The soluble glucose dehydrogenase (sGDH) from Acinetobacter calcoaceticus has been widely studied and is used, in biosensors, to detect the presence of glucose, taking advantage of its high turnover and insensitivity to molecular oxygen. However, this dimeric enzyme, composed of two identical 453 amino acid monomers (pI = 8.75), also presents drawbacks in terms of broad substrate specificity and loss of activity over time. Briefly, all crystal structures contained a tight dimer of sGDH in the asymmetric unit, the dimeric interface extending over 1110 Å2 being maintained by the presence of two calcium ions as described in Oubrie et al. interacting with the N262-D273 loop, referred to as the 4CD loop in the nomenclature of Oubrie et al.. 2Fobs-Fcalc electron density maps from the wild-type and both mutant structures all showed a different molecule instead of the PQQ-cofactor, corresponding to a PQQ modified cofactor, with the bond between C4 and C5 missing.

The active site of PQQ from the wild-type enzyme at pH 8. The density at 5 σ from a Polder Omit Map (PHENIX) is superimposed onto a model of cleaved PQQ. Residues close to the cofactor are labeled, and show little reorganization compared with the structures published by Oubrie et al. When compared with the structure in Figure 2, the cleavage of PQQ is clearly demonstrated and the pyrrole ring is seen to be almost perpendicular to the quinone. The absence of this C-C bond permits a large rotation of the pyrrole ring (110° ± 2°) to assume a completely different conformation. Electron density is observed directly above the cleaved quinone, which could possibly be attributed to a molecule of H2O2, although there is no direct evidence to substantiate this hypothesis. Consequently, this density has intentionally been left unmodeled in the refined structure. The crystals were subjected to a relatively modest dose of X-ray during data collection, estimated (from the measured beam flux, the exposure time and the crystal volume) as 2.75 MGy for the single and double mutant crystals and 0.9 MGy for the very high-resolution wild-type crystal. Third, a data set of the wild-type recorded on a rotating anode X-ray generator at a slightly lower resolution, on a similar crystal and an absorbed dose of around 0.1 MGy, displayed the same bond cleavage. Taken together, these points strongly suggest that the cleavage of PQQ is not caused by direct radiation damage by the X-ray beam. A notable decline was observed in the absorbance at 340 nm, indicative of enzyme activity, with a 5-fold decrease for the Y343F mutant and a 1.4-fold decrease for the wild-type enzyme over 6 h. Specifically, activity losses of 60% for the wild-type and 30% for the Y343F mutant were recorded after 8 h at 25°C. Notably, alterations to the disulfide bridge were not detected using dithionitrobenzoate (DTNB), a reagent selectively reactive toward free thiol groups.

>[2x]DVPLTPSQFAKAKSENFDKKVILSNLNKPHALLWGPDNQIWLTERATGKILRVNPESGSVKTVFQVPEIVNDADGQNGLLGFAFHPDFKNNPYIYISGTFKNPKSTDKELPNQTIIRRYTYNKSTDTLEKPVDLLAGLPSSKDHQSGRLVIGPDQKIYYTIGDQGRNQLAYLFLPNQAQHTPTQQELNGKDYHTYMGKVLRLNLDGSIPKDNPSFNGVVSHIYTLGHRNPQGLAFTPNGKLLQSEQGPNSDDEINLIVKGGNYGWPNVAGYKDDSGYAYANYSAAANKSIKDLAQNGVKVAAGVPVTKESEWTGKNFVPPLKTLYTVQDTYNYNDPTCGEMTYICWPTVAPSSAYVYKGGKKAITGWENTLLVPSLKRGVIFRIKLDPTYSTTYDDAVPMFKSNNRYRDVIASPDGNVLYVLTDTAGNVQKDDGSVTNTLENPGSLIKFTYKAK>MHHHHHHKNIVNTSILSIVYKKDDLIDLSRYGAKINIGDRVYYDSIDKNQIKLINLESSTIEVILKNAIVYNSMYENFSTSFWIKIPKYFSKINLNNEYTIINCIENNSGWKVSLNYGEIIWTLQDNKQNIQRVVFKYSQMVNISDYINRWIFVTITNNRLTKSKIYINGRLIDQKPISNLGNIHASNKIMFKLDGCRDPRRYIMIKYFNLFDKELNEKEIKDLYDSQSNSGILKDFWGNYLQYDKPYYMLNLFDPNKYVDVNNIGIRGYMYLKGPRGSVVTTNIYLNSTLYEGTKFIIKKYASGNEDNIVRNNDRVYINVVVKNKEYRLATNASQAGVEKILSALEIPDVGNLSQVVVMKSKDDQGIRNKCKMNLQDNNGNDIGFIGFHLYDNIAKLVASNWYNRQVGKASRTFGCSW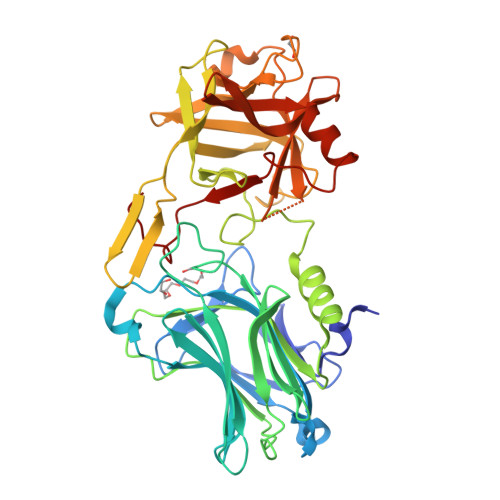EFIPVDDGWGESSL[2x]> MQSLEKQSSKGQWLTTWATAPQLVEPKNLPPEPGLSGNTLRQIVRVSVGGKKLRLRFSNKYSMDSLAVKAVSIAVPSDSSNVDAATIRSLTFEKKNNFKIAPGSDIYSDEVNFNLKPNSLLAITVSYAKVTQSVTGHPASRTTSFIVKGEQTNAEVFKNPVKTDHWYSLFNIDVKT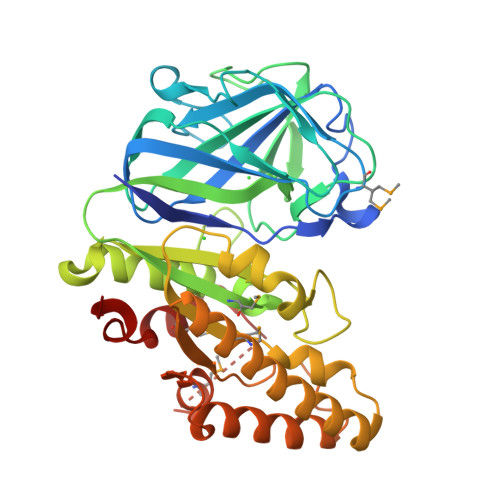SEPSYAVAIMGNSITDGRGSGTNRQNRWPDIFSQRLLANPSTRNISVLNLGIGGNCVVRGGLGPTALDRFDYNILNQQGVKWLIILEGVNDLGGTRDPDDASKRTEELIAAYQVMIDKAHANGIKVYGATILPFGKSFYEKPFRIEEWKKVNDWIRNSGKFDAVIDFAKHMQSENPEVILNDMHDHDFLHPNEAGYRRMGEFVDLNLFKNE>[2x]MTMDEQQSQAVAPVYVGGFLARYDQSPDEAE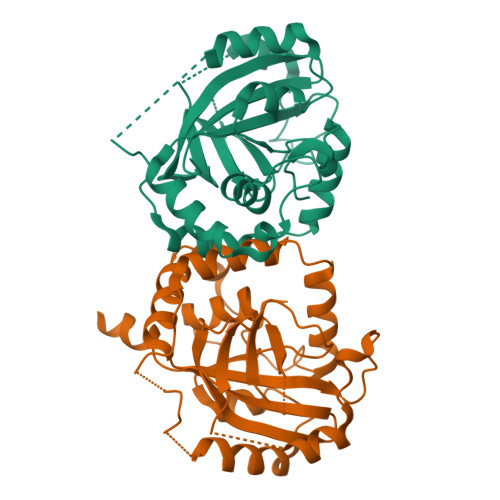LLLPRDVVEHWLHAQGQGQPSLSVALPLNINHDDTAVVGHVAAMQSVRDGLFCLGCVTSPRFLEIVRRASEKSELVSRGPVSPLQPDKVVEFLSGSYAGLSLASRRCDDVEQATSLSGSETTPFKHVALCSVGRRRGTLAVYGRDPEWVTQRFPDLTAADRDGLRAQWQRCGSTAVDASGDPFRSDSYGLLGNSVDALYIRERLPKLRYDKQLVGVTERESYVKA>AIPSSLSINWNNYATGAYSSGNAASDFGNAGGWNQSRSYISDGTLRVTLLKNALSGAGGLISNIDVSDGTEYELDYDVRFHSQFDWSRGGAVGFGFSIGEGNTGGDPGWDGNGGTLRMAWYQTDAGRVFFQPYIYHKDQPGQYGDTFGKSYPSSGSIT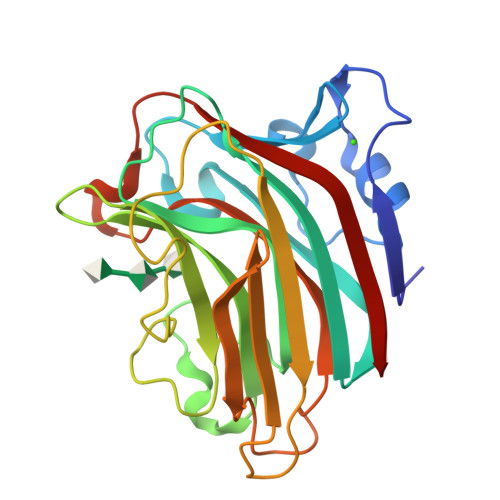KGTTYHVHVYIKSNTGSNRDGRAQIIINGTTVLDTAIRWTTNDAQRLIKNMTFHTFRGGSQTYWQSPVDSYIYYDNLVLRKIR[3x]>MGTKNIGKGLTFEDI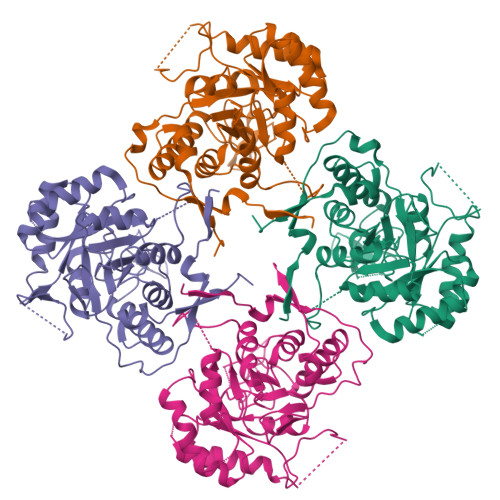LLVPNYSEVLPREVSLETKLTKNVSLKIPLISSAMDTVTEHLMAVGMARLGGIGIIHKNMDMESQVNEVLKVKNWISNLEKNESTPDQNLDKESTDGKDTKSNNNIDAYSNENLDNKGRLRVGAAIGVNEIERAKLLVEAGVDVIVLDSAHGHSLNIIRTLKEIKSKMNIDVIVGNVVTEEATKELIENGADGIKVGIGPGSICTTRIVAGVGVPQITAIEKCSSVASKFGIPIIADGGIRYSGDIGKALAVGASSVMIGSILAGTEESPGEKELIGDTVYKYYRGMGSVGAMKSGSGDRYFQEKRPENKMVPEGIEGRVKYKGEMEGVVYQLVGGLRSCMGYLGSASIEELWKKSSYVEITTSGLRESHVHDVEIVKEVMNYSK[4x]>[6x]MPGKILLLNGPNLNMLGKAEPDIYGHDTLEDVVALATA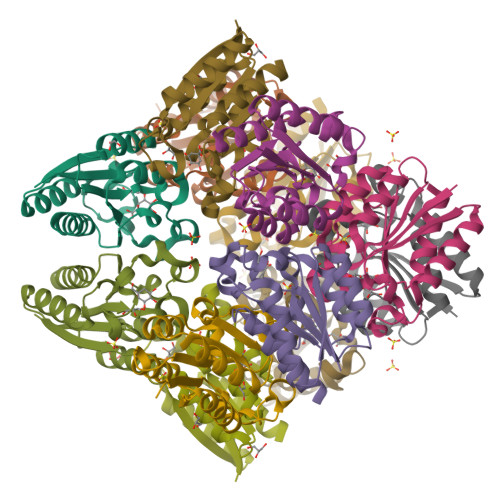EAAKHGLEVEALQSNHEGELIDALHNARGTHIGCVINPGGLTHTSVALLDAVKASELPTVEVHISNPHAREEFRHHSYISLAAVSVIAGAGIQGYRFAVDILANLKKLEHHHHHH>[6x]MVKSRKISILLAVAMLVSIMIPTTAFAGPTKAPTKDGTSYKDLFLELYGKIKDPKNGYFSPDEGIPYHSIETLIVEAPDYGHVTTSEAFSYYVWLEAMYGNLTGNWSGVETAWKVMEDWIIPDSTEQPGMSSYNPN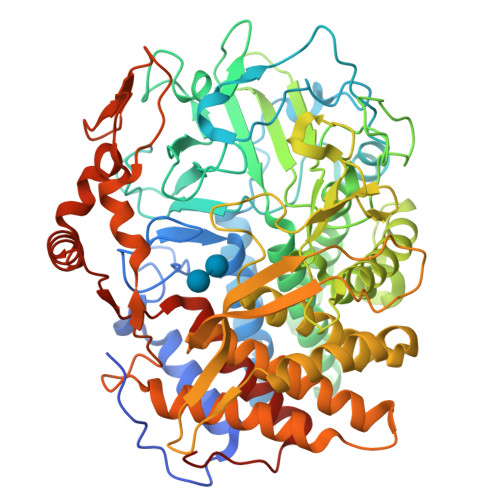SPATYADEYEDPSYYPSELKFDTVRVGSDPVHNDLVSAYGPNMYLMHWLMDVDNWYGFGTGTRATFINTFQRGEQESTWETIPHPSIEEFKYGGPNGFLDLFTKDRSYAKQWRYTNAPDAEGRAIQAVYWANKWAKEQGKGSAVASVVSKAAKMGDFLRNDMFDKYFMKIGAQDKTPATGYDSAHYLMAWYTAWGGGIGASWAWKIGCSHAHFGYQNPFQGWVSATQSDFAPKSSNGKRDWTTSYKRQLEFYQWLQSAEGGIAGGATNSWNGRYEKYPAGTSTFYGMAYVPHPVYADPGSNQWFGFQAWSMQRVMEYYLETGDSSVKNLIKKWVDWVMSEIKLYDDGTFAIPSDLEWSGQPDTWTGTYTGNPNLHVRVTSYGTDLGVAGSLANALATYAAATERWEGKLDTKARDMAAELVNRAWYNFYCSEGKGVVTEEARADYKRFFEQEVYVPAGWSGTMPNGDKIQPGIKFIDIRTKYRQDPYYDIVYQAYLRGEAPVLNYHRFWHEVDLAVAMGVLATYFPDMTYKVPGTPSTKLYG Some Gram-negative bacteria target their competitors by exploiting the type VI secretion system to extrude toxic effector proteins. To prevent self-harm, these bacteria also produce highly specific immunity proteins that neutralize these antagonistic effectors. The opportunistic pathogen Serratia marcescens has recently been shown to utilize T6-dependent secretion of two family 4 amidases, Ssp1 and Ssp2, to mediate antibacterial activity. In S. marcescens, the resistance-associated proteins Rap1a and Rap2a neutralize Ssp1 and Ssp2, respectively.

The Rap1a subunit displays a compact globular structure constructed from five α-helices that assemble to form the highly stable symmetric dimer that constitutes the asymmetric unit. This is consistent with the size-exclusion chromatography data, which identified that only a dimer was observed in solution. The NCS is highly conserved, with an r.m.s.d. of 0.6 Å for a least-squares overlay of 96 Cα positions. A disulfide bond is formed between Cys78 (in the α2–α3 loop) and Cys122 in the C-terminal region. This interaction appears to be crucial to stabilizing the subunit fold since it helps position α2, α3 and α5 close to each other and these segments of secondary structure provide the side chains that form the hydrophobic core of the subunit. During initial recombinant expression tests it was noted that soluble protein was only produced in E. coli Rosetta-gami (DE3) cells, a strain that promotes the formation of disulfide bonds in the cytoplasm and so mimics what might occur in the oxidative environment of the periplasm. This suggests that the covalent bond is necessary for correct folding to occur and for stability of the Rap1a fold and dimeric quaternary structure. Interactions involving residues in α2 make the major contribution to dimer formation. Each subunit contributes a surface area of 1130 Å2 to the dimer interface, which is 20% of the solvent-accessible surface area (ASA) of the subunit (5700 Å2). We therefore conclude that the Rap1a fold has not been observed previously, making it a unique member of the T6SS immunity family of proteins. In Rap1a, the segment linking α2 and α3, residues 74–84, shows high average B factors (temperature factors; 76.4 Å2) compared with the overall average B factor (31.5 Å2) and relatively diffuse electron density.

>[2x]GHMEQTSIAHLTSDDVNLPGSDFFRFYRSADKQEKEKARIYLLGVLDATEGKSWCQYSQLQTVTLQEFVFEFFNKLPAARLHERAAPLIEEALATRFPCKGGKA> MASPIESARIGEVKRETKQTNVSVKINLDGHGVSDSSTGIPFLDHMLDQLASHGLFDVHVRATGDTHIDDHHTNEDVALAIGTALLKA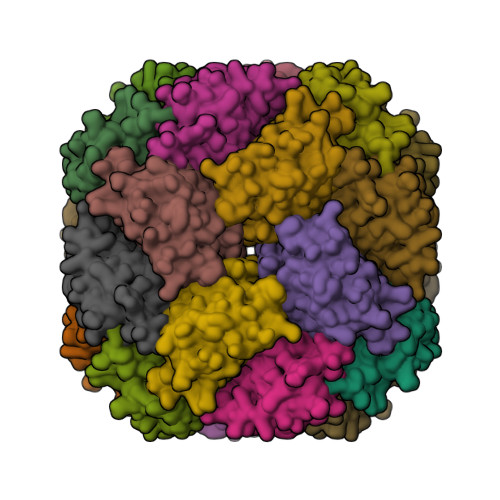LGERKGINRFGDFTAPLDEALIHVSLDLSGRPYLGYNLEIPTQRVGTYDTQLVEHFFQSLVNTSGMTLHIRQLAGKNSHHIIEATFKAFARALRQATESDPRRGGTIPSSKGVLSRS>[6x]GASKKSAAEASKKPRQKRTATKAYN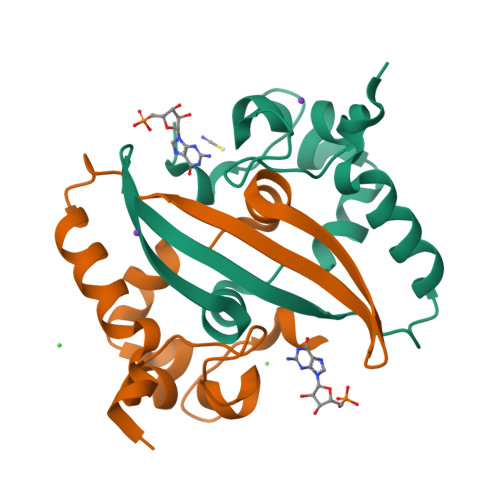VTQAFGRRGPEQTQGNFGDQELIRQGTDYKHWPQIAQFAPSASAFFGMSRIGMEVTPSGTWLTYTGAIKLDDKDPNFKDQVILLNKHIDAYKTFP[(1S)-1,2,3,4-tetrahydroisoquinolin-1-yl]methanol 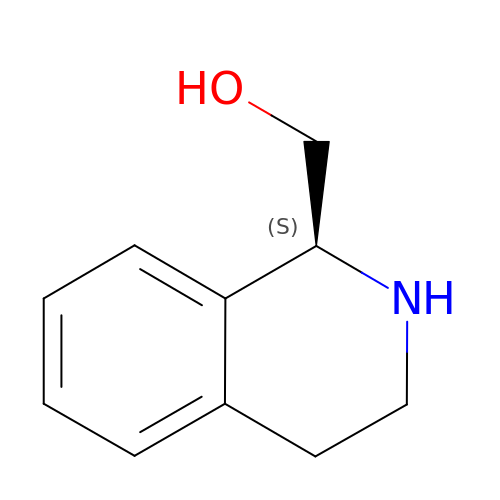| C10 H13 N O | BGGIPVPHBWWEJT-SNVBAGLBSA-N[(2~{S})-2,3-bis(oxidanyl)propyl] (~{E})-undec-2-enoate 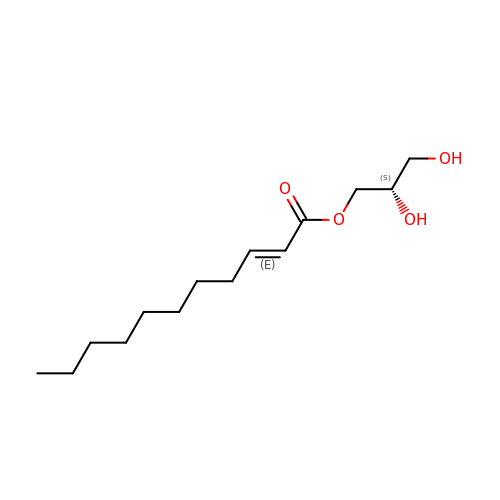| C14 H26 O4 | INMIULFREHIAOX-LXKVQUBZSA-N> EAASSSDADGKEVGSSGEGNRATGGKWRRPSLAQQRARRAQLPPAFDVVHWNDEDISRGHLLRVLHRDTFVVLDYH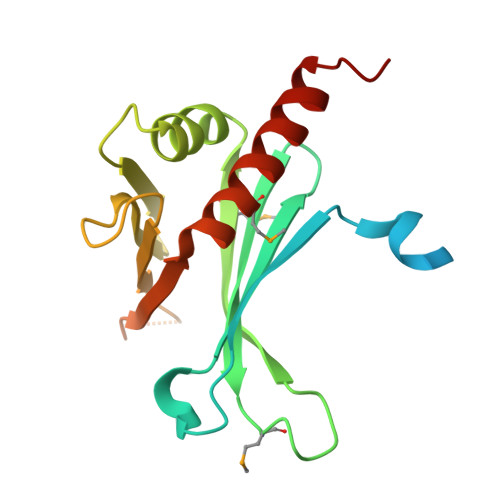RQARMLTEEGNKAERVVSVMLPAVYTARFLAVLEGRSEKVEVHSRYTNATFTPNPAAPYTFTLKCTSTRPAQQKQQVAGEEGDETFEWTVEFDVAESLMLQRFLTQALHYNTGFARTSV(4S)-N-((3R,5R)-1-(cyclopropanecarbonyl)-5-((5-(phenylethynyl)thiophene-2-carboxamido)methyl)pyrrolidin-3-yl)-4-fluoropyrrolidine-2-carboxamide | 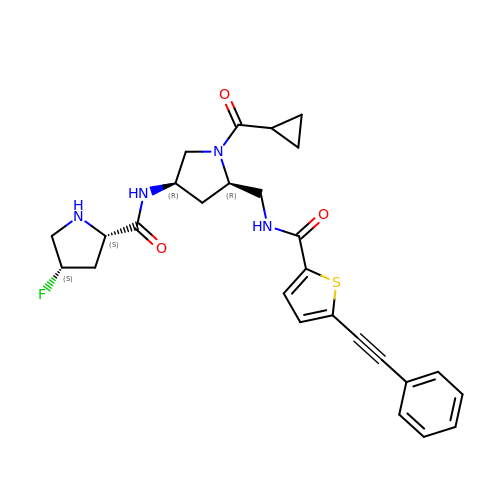C27 H29 F N4 O3 S | ZFFWZIADZMCJNF-GNXKAVGDSA-N As part of our structural genomics effort in targeting novel protein families, we determined crystal structures of three bacterial proteins from a previously structurally uncharacterized protein family Pfam PF08000 [also known as domain of unknown function family 1696 (DUF1696)],11 which appears to be involved in the bacterial cell envelope stress response. These structures share a common domain that is surprisingly similar to the eukaryotic PH-like domains, thus providing the first direct evidence for the existence of PH-like domains in prokaryotes. PHb1 and PHb2 share a common domain that is structurally similar to eukaryotic PH domains, which we have defined as a PHb domain (PH domain in bacteria). The PHb proteins form oligomeric ring assemblies of different sizes and symmetries, providing an excellent example of how molecular architecture can evolve, where the general form of the molecular assembly is preserved, but its size is expandable.

To our surprise, these structures had similarity to eukaryotic PH-like domains that we now define as bacterial PH domain-like proteins from group 1 (PHb1) {S. loihica [PHb1(sl), residues 9–124] and S. amazonensis [PHb1(sa), residues 1–125]} and from group 2 (PHb2) [E. sibiricum 255-15 (PHb2, residues 13–204)]. PHb1(sl) (residues 9–124) has only a single PHb domain that consists of the canonical seven β-strands in two β-sheets (β1–β4 and β5–β7) and a C-terminal helix (α1). It has an additional short β-strand β0 that connects to β1 with a large loop containing helix α0 that packs against the β1–β4 surface. The final model of PHb1(sl) contains 561 amino acid residues, 1 chloride ion, 7 (4S)-2-methyl-2,4-pentanediols, and 322 waters in the asu. PHb1(sl) and PHb1(sa) form a disk with non-crystallographic C5 symmetry that is normally only encountered in viruses with icosahedral capsids. The PHb1(sl) pentamer buries a total surface area of 9080 Å2 (34% of total surface area, 1816 Å2 per monomer). The formation of the pentamer in PHb1(sl) is mediated primarily through hydrogen-bonding interactions. β4 and β5 of two adjacent protomers form an antiparallel β-sheet, consisting of five hydrogen bonds between their main-chain atoms. As a result, the β0–β4 and β5–β7 of the next protomer form an extended eight-stranded β-sheet, arranged like the blades of a propeller (β-blade) at the base of the pentamer. The second contact point in the pentamer involves α1 (residues 113–121) from one monomer and the 310 helix region (residues 25–29) of the adjacent protomer. In PHb1(sl), these residues include Asp42 from β2, Asp55 and Gln57 from β3, and Lys63 from β4, as well as residues from the adjacent protomer: Glu80 from β5 and Asp86, Asp88, and Glu90 from β6.

>GGNAAEVNLDELAQELGPIMGDNEQLALAYRVIRDMFVFTNKRLILIDKQGVTGKKVSYHSVPYKAITHFEVETAGTFDMDAELKLWISGQKDPLVKELKKGTDVVGIQKTIANFSL[5x]> GSNVLTVYSPYQSNLIRPILNEFEKQEHVKIEIKHGSTQVLLSNLHNEDFSERGDVFMGGVLSETIDHPEDFVPYQDTSVTQQLEDYRSNNKYVTSFLLMPTVIVVNSDLQGDIKIRGYQDLLQPILKGKIAYSNPNTTTTGYQHMRAIYSMHHRVSDVHQFQNHAMQLSKTSKVIEDVAKGKYYAGLSYEQDARTWKNKGYPVSIVYPIEGTMLNVDGIALVKNAHPHPKRKKLVQYLTSRSVQQRLVAEF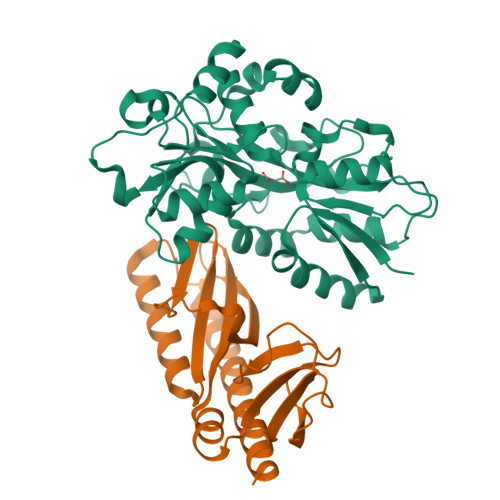DAKSIRKDVSEQSDQSIENLKNIPLIPKSKLPDIPHHKFLEMIQ;> TIHQHVDESQSSLHHTEKQIQTFITQHNNSFQELDLTNHHDVTATKRELLKLIHQQPATLYYELSGPNQFITNNYEHLNTKNMYLFSTHQLKFKNSTYMLKIYMANTPRLSEIKKDNRQFALIVDQYDNILYANDDRFTIGEKYRPQQFGFMNESVKLNHADHRLIIYKDI>[2x]MVSLRLPLILLSLLAISFSCSAAPPPVYDT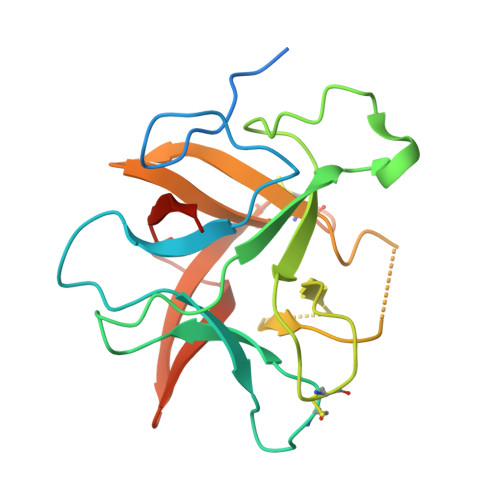EGHELSADGSYYVLPASPGHGGGLTMAPRVLPCPLLVAQETDERRKGFPVRFTPWGGAAAPEDRTIRVSTDVRIRFNAATICVQSTEWHVGDEPLTGARRVVTGPLIGPSPSGRENAFRVEKYGGGYKLVSCRDSCQDLGVSRDGARAWLGASQPPHVVVFKKARPSPPE> MTKQEKTALNMARFIRSQTLTLLEKLNELADAADEQAD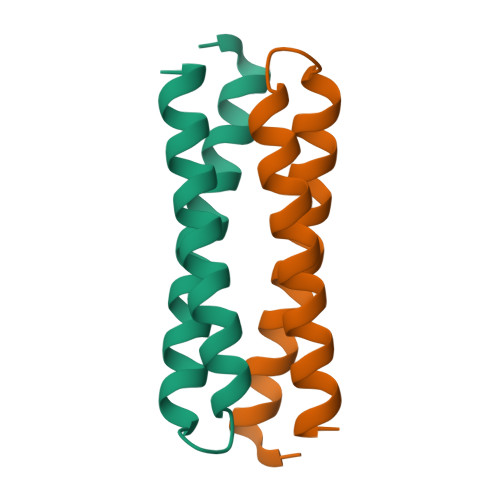ICESLHDHADELYRSCLARFGDDGENL> AH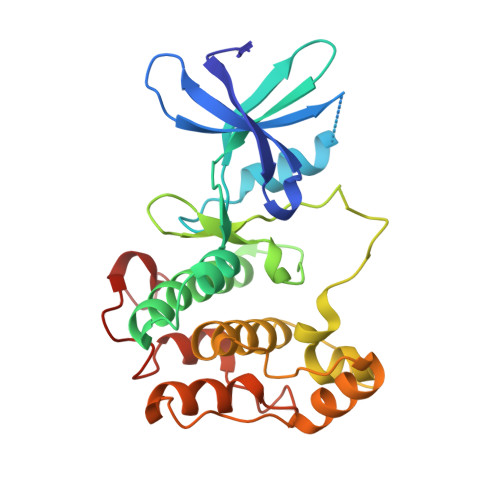IGNYQIVKTLGEGSFGKVKLAYHTTTGQKVALKIINKKVLAKSDMQGRIEREISYLRLLRHPHIIKLYDVIKSKDEIIMVIEYAGNELFDYIVQRDKMSEQEARRFFQQIISAVEYCHRHKIVHRDLKPENLLLDEHLNVKIADFGLSNIMTDGNFLKTSCGSPNYAAPEVISGKLYAGPEVDVWSCGVILYVMLCRRLPFDDESIPVLFKNISNGVYTLPKFLSPGAAGLIKRMLIVNPLNRISIHEIMQDDWFKVDLPEYLLPPDLK> MVSNWNWSGKKGRRTPRRGYTRPFKSAVPTTRVVVHQSAVLKKDDVSGSEIKPEGDVARYKIRKVMLSCTLRMRPGELVNYLIVKCSSPIVNWSAAFTAPALMVKESCQDMITIIGKGKVESNGVAGSDCTKSFNKFIRLGAGISQTQHLYVVMYTSEAVKTVLEHRVYIEV

Nanoviruses are plant multipartite viruses with a genome composed of six to eight circular single-stranded DNA segments. Segment S encodes the capsid protein (CP) that assembles into virus particles, which encapsidate individually single DNA segments. The distinct genome segments are encapsidated individually in icosahedral particles that measure ≈18 nm in diameter. Here, we address this question by reporting a structural characterisation of the FBNSV particles at quasi-atomic resolution (3.2 Å) by cryogenic-electron-microscopy (cryo-EM) single-particle analysis.

Image processing of the best resolved 3D classes enabled us to compute a 3D map of the FBNSV electron scattering density—with imposed icosahedral symmetry—(Electron Microscopy Data Bank entry EMD-10097) from 5,156 non-binned (1.21 Å/pixel) selected particles at an average resolution of 3.2 Å. The highly positively-charged N-terminal stretch (residues 1 to 26) of the CP, which is predicted to be dynamically flexible and likely buried within the genetic material at the interior of the viral particles, is not visible in the reconstructed density and thus not included in the deposited atomic model. The CP fold is a typical wedge-shaped jelly-roll domain—the most prevalent fold among viral CPs —composed by two packed, four-stranded, anti-parallel β-sheets (named BIDG and CHEF according to classic labelling of jelly-roll β-strands using letters B through I). Each jelly-roll subunit is oriented so that the lateral sides of two β-strands (F and G) face the capsid interior and the closest fivefold axis, while the two strands (B and C) on the opposite side of the jelly-roll contribute to the outer surface of the capsid. The CP subunits interact with each other most extensively at the interfaces generated by the icosahedral fivefold symmetry axes (subunit-subunit interface area: 950 Å2), where the BIDG sheet of each subunit is tightly packed against part of the CHEF sheet and the intervening EF connection of an adjacent subunit. Fewer interactions are observed at the twofold interfaces (interface area: 393 Å2). These involve loops at the base of the wedge, including the two serines (residues 87 and 88) at the beginning of the EF connection. The fewest contacts between subunits are found at the threefold interfaces (interface area: 301 Å2) and involve the first visible residues of the N-terminal stretch, which appear to emerge from the capsid interior, the adjacent C-terminal stretch, which points towards the capsid interior, and two loops at the base of the jelly-roll wedge. Though less resolved (>4.5 Å) than the density of the surrounding protein layer, the residual genome density is comparably strong in the neighbourhoods of the CP-CP fivefold interfaces, where a putative aromatic base—sandwiched between the BIDG and CHEF sheets of neighbouring CP subunits—protrudes towards the main-chain atoms of residues 102 to 104 of the EF connection.>MDTGSSEPDANRCPSQRSSHALQTLTTRRAVRAFADRPVDDSLLDPMLDAMLAAPSASNKQAWAFVAVRERRALRLLRAFSPGIIELPPLVVAACFDRSRAVGGSGNSTDSGDSWDEGMLCVAMAVENLLLAAHCLGLGGCPSGSFRRGPVRRLLGLPDHLEPLLLVPIGHPARPLAPAPRRDRNEVVSHERWGTGSS[2x];>[4x]MSAGEPEVRQVGEELLLLAAYLLSSGRGLLDEPRQYGTFRCLDAARRVLALAAGTGPHHPELDALRGRMDDVMCGPMGDHELDTLLDQMCERLATVLEDPDVISD

Here, we determined the structure and mechanism of the cyclodipeptide oxidase from the halophile Nocardiopsis dassonvillei (NdasCDO), a component of the biosynthetic pathway for nocazine natural products. We demonstrated that NdasCDO forms filaments in solution, with a covalently bound flavin mononucleotide (FMN) cofactor at the interface between three distinct subunits. The enzyme exhibits promiscuity, processing various cyclic dipeptides as substrates in a distributive manner. CDOs enable the facile incorporation of a Cα-Cβ double bond into the 2,5-diketopiperazine backbone.

To gain insights into the structural organisation of NdasCDO, we performed helical reconstruction from the cryo electron microscopy data collected from a cryo vitrified grid containing ordered NdasCDO filaments to resolve a 3.0 Å resolution map. The filament was composed of alternating repeating units of homodimers of NdasCDO subunit A (NdasCDO-A) and homodimers of NdasCDO subunit B (NdasCDO-B), such that the interface between the two homodimers constitutes the heterotetrametric form of the molecule representing the biologically relevant asymmetric unit. Continuous filament is formed by shifting the homotetramer along the screw axis with helical rise of 45.45 Å, helical twist of 132.37° and overall helical pitch of 123.6 Å. NdasCDO-A was composed of four anti-parallel beta strands surrounded by five alpha helical elements. Subunit B: NdasCDO-B is an α-helical protein composed of 4 antiparallel helices and, together with the second monomer, forms a dimeric 8-helical bundle structure. The FMN cofactor is covalently attached to Cys121 from subunit A through an 8α-S-cysteinyl linkage and sandwiched between subunits A and B. In comparison, the same residues were observed in NdasCDO including R32, N59 and S145 from NdasCDO-A and E32, P33, Y36, and R40 from NdasCDO-B. Whilst R32 is in close proximity to one of the C2 carbonyl groups from FMN’s isoalloxazine ring, R28, R29 and R181 also participate in polar interactions with the phosphate group of FMN. However, Glu117 is 7 Å from Ser58-A or Tyr36-B, too far for a direct interaction but nevertheless in a position that could lead to interactions with CDP substrates and their side chains to allow proton transfer with the cofactor. Together Tyr36-B, Phe39-B and Met77-B could limit access to the substrate binding site and FMN, as the bulky side chains obstruct the active site. The FMN and substrate binding pocket are in a deep cavity, mostly surrounded by positively charged and hydrophobic residues, and further shielded from solvent by Tyr36-B, Phe39-B and Met77-B. The active site of NdasCDO comprises residues from two A subunits and one B subunit, providing functional rationale for its occurrence as a filament.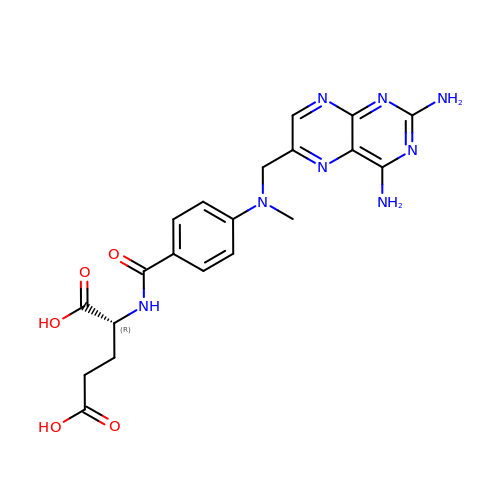(2~{R})-2-[[4-[[2,4-bis(azanyl)pteridin-6-yl]methyl-methyl-amino]phenyl]carbonylamino]pentanedioic acid | C20 H22 N8 O5 | FBOZXECLQNJBKD-CYBMUJFWSA-N> LTNLVAEPFAKLEQDFGGSIGVYAMDTGSGATVSYRAEERFPLCSSFKGFLAAAVLARSQQQAGLLDTPIRYGKNALVPWSPISEKYLTTGMTVAELSAAAVQYSDNAAANLLLKELGGPAGLTAFMRSIGDTTFRLDRWELELNSAIPGDARDTSSPRAVTESLQKLTLGSALAAPQRQQFVDWLKGNTTGNHRIRAAVPADWAVGDKTGTCGVYGTANDYAVVWPTGRAPIVLAV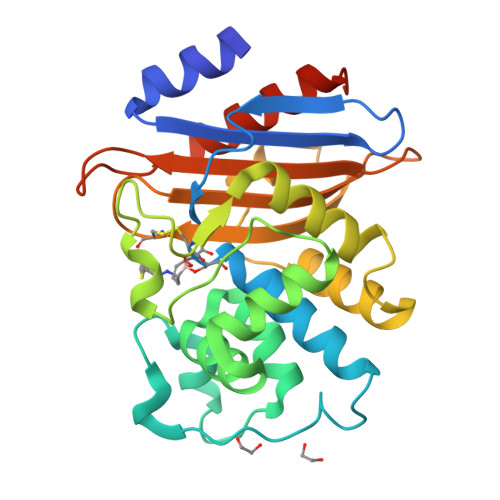YTRAPNKDDKHSEAVIAAAARLALEGLGVNGQCEHHHHHH> MNVGTAHSEVNPNTRVMNSR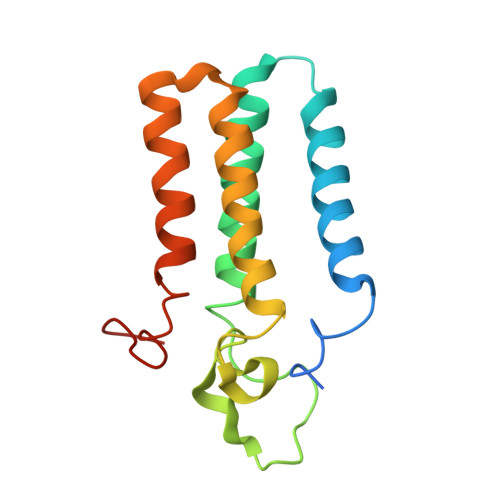GIWLSYVLAIGLLHIVLLSIPFVSVPVVWTLTNLIHNMGMYIFLHTVKGTPFETPDQGKARLLTHWEQMDYGVQFTASRKFLTITPIVLYFLTSFYTKYDQIHFVLNTVSLMSVLIPKLPQLHGVRIFGINKY> SPDKQMAVLPRRERNRQAAAANPENSRGKGRRGQRGKNRGCVLTA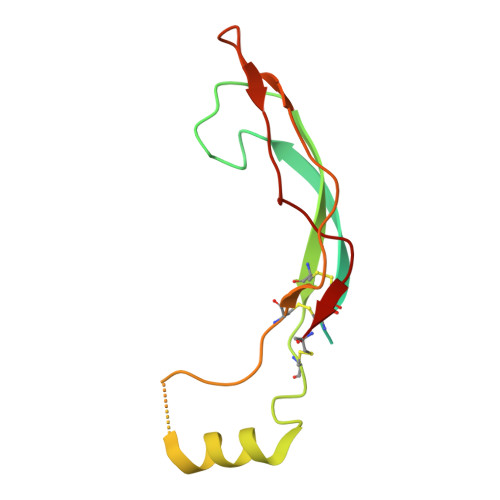IHLNVTDLGLGYETKEELIFRYCSGSCDAAETTYDKILKNLSRNRRLVSDKVGQACCRPIAFDDDLSFLDDNLVYHILRKHSAKRCGCI>GPLGSMSQSNRELVVDFLSYKLSQKGYSWSQMAAVKQALREAGDEFELRYRRAFSDLTSQLHITPGTAYQSFEQVVNELFRDGVNWGRIVAFFSFGGALCVESVDK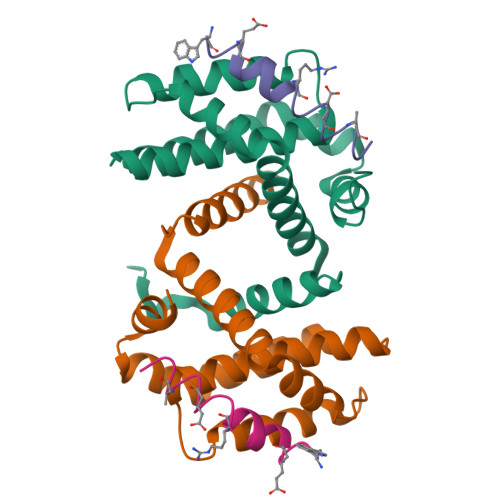EMQVLVSRIAAWMATYLNDHLEPWIQENGGWDTFVELYGNNAAAESRKGQER[2x];>[2x]XWAREIGAXLRRMADDLNAQYEX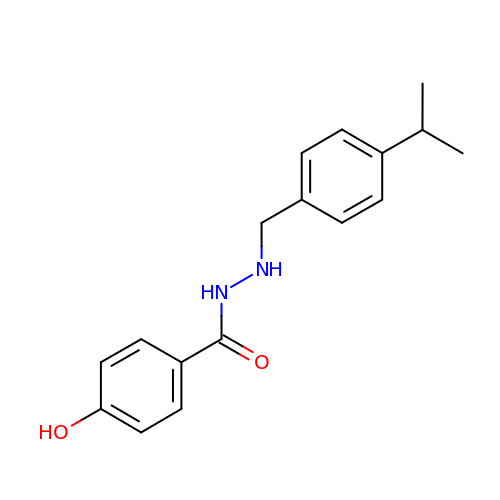4-HYDROXY-N'-(4-ISOPROPYLBENZYL)BENZOHYDRAZIDE | C17 H20 N2 O2 | MFDXHRPPSJRQFX-UHFFFAOYSA-N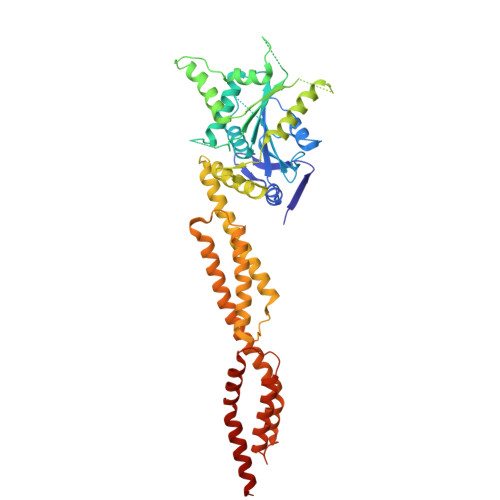>[4x]SMALEIHMSDPMCLIENFNEQLKVNQEALEILSAITQPVVVVAIVGLYRTGKSYLMNKLAGKNKGFSVASTVQSHTKGIWIWCVPHPNWPNHTLVLLDTEGLGDVEKADNKNDIQIFALALLLSSTFVYNTVNKIDQGAIDLLHNVTELTDLLKARNSPDLDRVEDPADSASFFPDLVWTLRDFCLGLEIDGQLVTPDEYLENSLRPKQGSDQRVQNFNLPRLCIQKFFPKKKCFIFDLPAHQKKLAQLETLPDDELEPEFVQQVTEFCSYIFSHSMTKTLPGGIMVNGSRLKNLVLTYVNAISSGDLPCIENAVLALAQRENSAAVQKAIAHYDQQMGQKVQLPMETLQELLDLHATSEREAIEVFMKNSFKDVDQSFQKELETLLDAKQNDICKRNLEASSDYCSALLKDIFGPLEEAVKQGIYSKPGGHNLFIQKTEELKAKYYREPRKGIQAEEVLQKYLKSKESVSHAILQTDQALTETEKK> MRMSDGAAPKANGSEASGQDLVPTAVEQAVPIQPVAGSALAAPAAGQINQIDPWIFQNFVQCPLGEFSISPRNTPGEILFDLALGPGLNPYLAHLSAMYTGWVGNMEVQLVLAGNAFTAGKVVVALVPPYFPKGSLTTAQITCFPHVMCDVRTLEPIQLPLLDVRRVLWHATQDQEESMRLVCMLYTPLRTNSPGDESFVVSGRLLSKPAADFNFVYLTPPIERTIYRMVDLPVLQPRLCTHARWPAPIYGLLVDPSLPSNPQWQNGRVHVD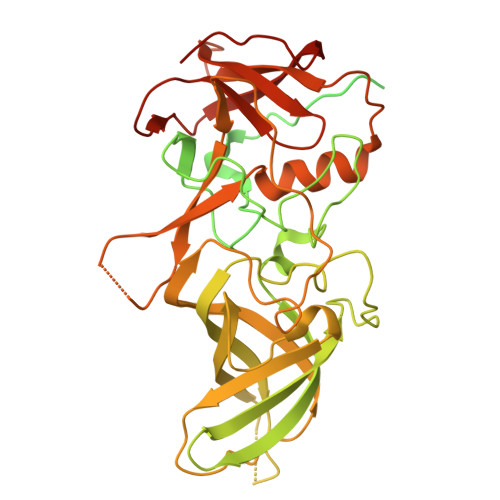GTLLGTTPVSGSWVSCFAAEAAYEFQSGTGEVATFTLIEQDGSAYVPGDRAAPLGYPDFSGQLEIEVQTETTKTGDKLKVTTFEMILGPTTNVDQAPYQGRVYASLTAVASLDLVDGRVRAVPRSIYGFQDVIPEYNDGLLVPLAPPIGPFLPGEVLLRFRTYMRQLDTADAAAEAIDCALPQEFISWFASNAFTVQSDALLLRYRNTLTGQLLFECKLYSEGYIALSYSGSGPLTFPTDGFFEVVSWVPRLFQLASVGSLTTGRTLKQ>[3x]MSAKVYFHETFENRDKWIDSTSSGKALGPFKIVSGKWYGDANNKGLQTSEDNKFYIAAAKLDEEFSNKDKNLIVQYNLKFEQGIDCGGGYIKLLPKKSIESEEKFTPESEYNIMFGPDVCGGSKRTHVIMNYKGKNNLIRKEIKCESDDISHLYTLIIRPNNTYVVKIDGVEKQEGKFDEDWDMLAPKEIDDGSGIANPDYVYDPELYKYDSFAYIGIDVWQVKAGTIYDDILITDDIEEAEKEAKVILERNAAEKKMRDEIKEAENGHHHHHH

Calreticulin (CRT) is a 46 kDa soluble multifunctional protein that was initially identified as an endoplasmic reticulum (ER) chaperone for monoglycosylated proteins and is also involved in Ca2+ regulation. Similar to its ER membrane homologue calnexin (CNX) ectodomain, CRT is composed of a globular domain, into which a flexible arm-like P (proline-rich) domain is inserted. The globular domain is made up of seven concave and six convex β-sheets forming a legume lectin fold. We have investigated the CRTs of two distinct parasites, Trypanosoma cruzi (TcCRT) and Entamoeba histolytica (EhCRT), for which a pathogenic role has been proposed.

E. histolytica is the causative agent of amoebiasis, a disease mainly characterized by dysentery that leads to about 100 000 deaths per year. During this process, EhCRT is exported from the ER to the phagolysosomal cupule, where it favours the phagocytosis process in a way similar to that described for human CRT on the surface of macrophages during the clearance of apoptotic cells. A similar EhCRT construct was then produced and beautiful crystals were obtained. The X-ray structures of the corresponding TcCRT and EhCRT constructs were solved using molecular replacement and refined to 2.45 and 2.15 Å resolution, respectively. A first example of a closed conformer is observed with EhCRT, and SAXS experiments conducted on TcCRT yielded new complementary insights into the dynamics of the flexible domains of CRT in solution. The first evidence is now provided of a complex conformational transition with the junction reoriented towards P-domain closure. Very intriguingly, a very reproducible electron density was observed within the GBS in the first EhCRT crystal form that was not related to the crystallization medium.> SSTVKTQSGSDVVADASADATGFPRQCGDYTVLGILTDNQDNSKAKENAETTLLRHPNVACLVGLWSQNTPMILAGLRSSDAIGKVAVVGFDEHPDTLAGIRDQSVYGTIVQQPYAFGYRSVQWLTTMAKGGEVEVPESGMIIIPHRSITGANVNEFAADIDAIKSGKGPILSGEQQIDGSGVRVAYITNSLDP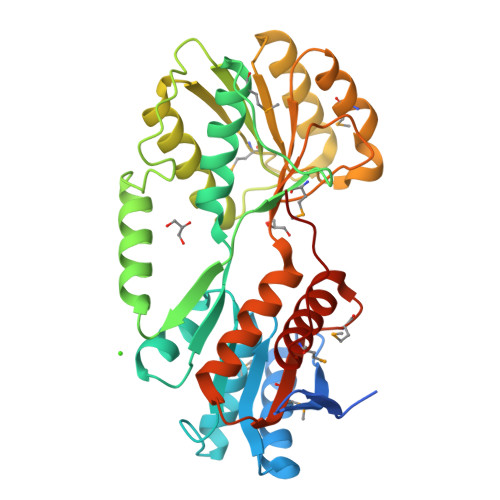FWTLADAGCKRAAEQFGCEVDVQMPSSGSIEEQKRFLESNVAAKVDGIAISPIDPENQVAMINDACKVTPVICQDSDAPASRRKFYLGTSNYLAGRAAGKLIQEAIPEGGEVMLFVGKMEVLNAQERSQGIMDELAGKPIPAILQGN N-((1S,2R)-3-(((1S)-2-(CYCLOHEXYLAMINO)-1-METHYL-2-OXOETHYL)AMINO)-2-HYDROXY-1-( PHENYLMETHYL)PROPYL)-3-((METHYLSULFONYL)(PHENYL)AMINO) BENZAMIDE 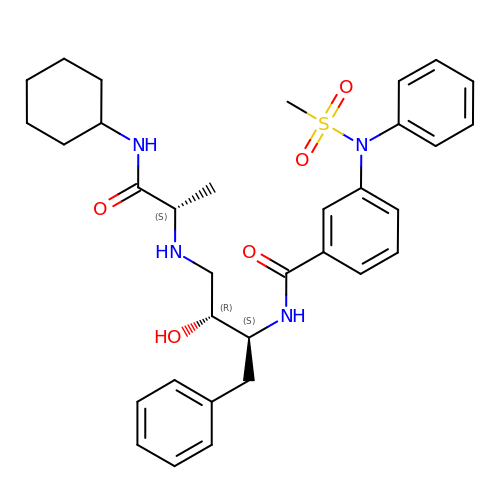| C33 H42 N4 O5 S | PSSKPAZTPVDDNS-RJSONGRPSA-N> SMPVAGSELPRRPLPPAAQERDAEPRPPHGELQYLGQIQHILRCGVRKDDRTGTGTLSVFGMQARYSLRDEFPLLTTKRVFWKGVLEELLWFIKGSTNAKELSSKGVKIWDANGSRDFLDSLGFSTREEGDLGPVYGFQWRHFGAEYRDMESDYSGQGVDQLQRVIDTIKTNPDD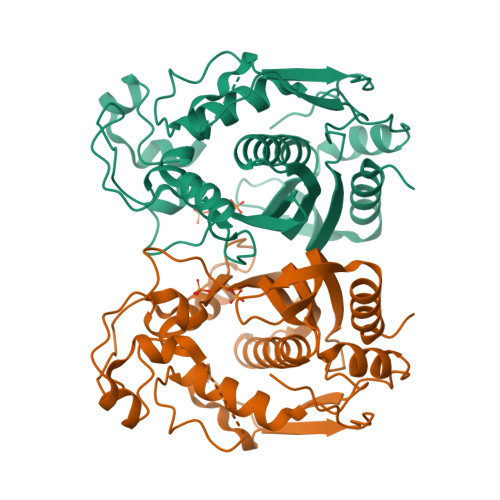RRIIMCAWNPRDLPLMKLPPCHALCQFYVVNSELSCQLYQRSGDMGLGVPFNIASYALLTYMIAHITGLKPGDFIHTLGDAHIYLNHIEPLKIQLQREPRPFPKLRILRKVEKIDDFKAEDFQIEGYNPHPTIKMEMAV>MQTVNEMLRRAATRAPDHCALAVPARGLRLTHAELRARVEAVAARLHADGLRPQQRVAVVAPNSADVVIAILALHRLGAVPALLNPRLKSAELAELIKRGEMTAAVIAVGRQVADAIFQSGSGARIIFLGDLVRDGEPYSYGPPIEDPQREPAQPAFIFYTSGTTGLPKAAIIPQRAAESRVLFMSTQVGLRHGRHNVVLGLMPLYHVVGFFAVLVAALALDGTYVVVEEFRPVDALQLVQQEQVTSLFATPTHLDALAAAAAHAGSSLKLDSLRHVTFAGATMPDAVLETVHQHLPGEKVNIYGTTEAMNSLYMRQPKTGTEMAPGFFSEVRIVRIGGGVDEIVANGEEGELIVAASDSAFVGYLNQPQATAEKLQDGWYRTSDVAVWTPEGTVRILGRVDDMIISGGENIHPSEIERVLGTAPGVTEVVVIGLADQRWGQSVTACVVPRLGETLSADALDTFCRSSELADFKRPKRYFILDQLPKNALNKVLRRQ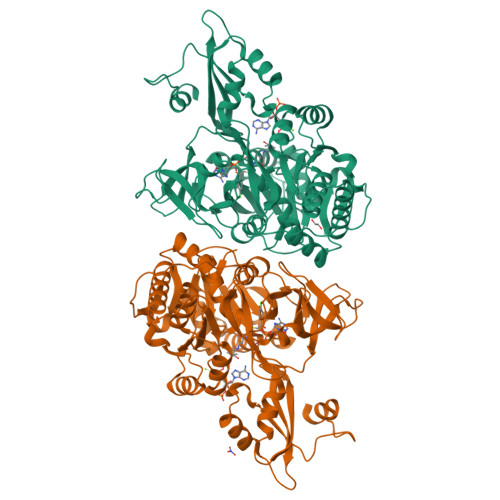LVQQVSS[2x]>[2x]MNTTPVHALTDIDGGIAVDPAPRLAGPPVFGGPGNDAFDLAPVRSTGREMLRFDFPGVSIGAAHYEEGPTGATVIHIPAGARTAVDARGGAVGLSGGYDFNHAICLAGGAGYGLEAGAGVSDALLERLEYRTGFAELQLVSSAVIYDFSARSTAVYPDKALGRAALEFAVPGEFPQGRAGAGMSASAGKVDWDRTEITGQGAAFRRLGDVRILAVVVPNPVGVIVDRAGT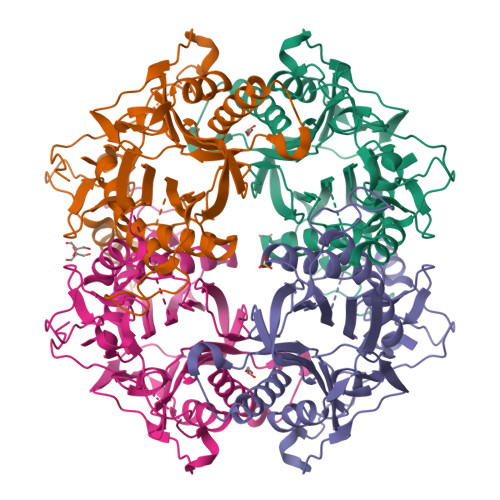VVRGNYDAQTGVRRHPVFDYQEAFAEQVPPVTEAGNTTISAIVTNVRMSPVELNQFAKQVHSSMHRGIQPFHTDMDGDTLFAVTTDEIDLPTTPGSSRGRLSVNATALGAIASEVMWDAVLEAGK>MVLYFIGLGLYDERDITVKGLEIAKKCDYVFAEFYTSLMAGTTLGRIQKLIGKEIRVLSREDVELNFENIVLPLAKENDVAFLTPGDPLVATTHAELRIRAKRAGVESYVIHAPSIYSAVGITGLHIYKFGKSATVAYPEGNWFPTSYYDVIKENAERG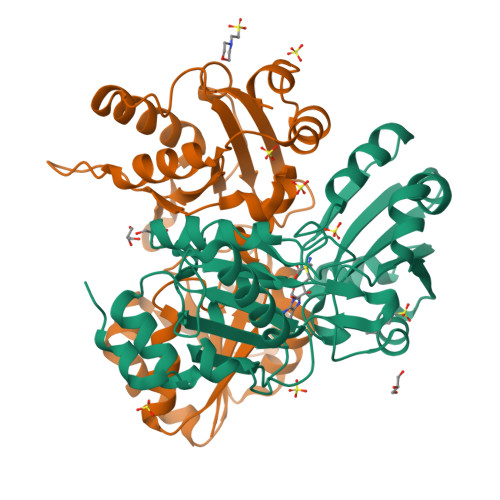LHTLLFLDIKAEKNMYMTANEAMELLLKVEDMKKGGVFTDDTLVVVLARAGSLNPTIRAGYVKDLIREDFGDPPHILIVPGKLHIVEAEYLVEIAGAPREILRVNV[2x]>MKTREIYAEMRCIPPVVLRADGRNFKNTLSGLGFEKPYDKTFARAMADTAELFIKKSGLSPLFAYTFSDEISFLFTDLPFDGRVEKIDSVVASFLGSALTIKLRLEEPIAFDSRLVALQKEEIPEYFHRRQLEAWRNFVASWGYYALRNEGMGRNEAAKYLKRKKESEIHEMLFERGINLATLPSWQRRGVIIS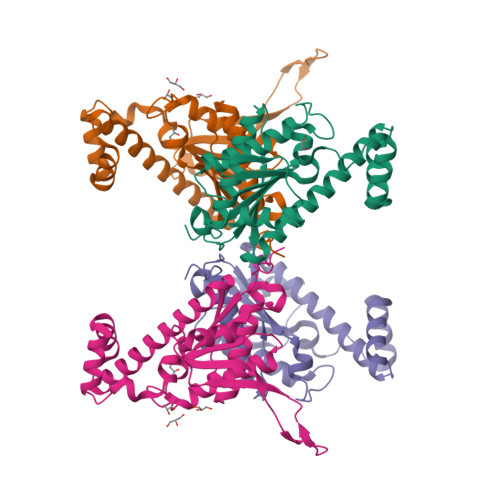KEAREIQGFNPVSGKEEKSLRRKITQNWEIPKFKSEKGIPFLEKLINRNLEHHHHHH[2x]> GSHLEPTQLGGLVTDQLARLCDVARLDRTDTETYVQTLATSLGTAAERSLALPPTTATLLSDDHTPVEYSLAFLPGATPALRVLVEPGWDSGDLAENGRAGLRAIRAMADRWNFSTDQLDLLEDLFFPVAPAGPFALWCALELRPGGVPGVKVYLNPAARGRDRRAETLREALDRLGHRQAFAALPPADDYPFLALDLGEWAAPRVKVYCTHESLSAQEAGEYSRLAAADGRDQTTDFFHAVAGTDAGGTGQPSTRRALTCHSFTDTVTGRPSGFTLHMPVRSYVEHDGRARDRAADVLRRYGMDNDALDRALAAVTPRPLDDGVGLVAYVALVHQLGRDPRVTVYVSSEAYAVQPPRTALA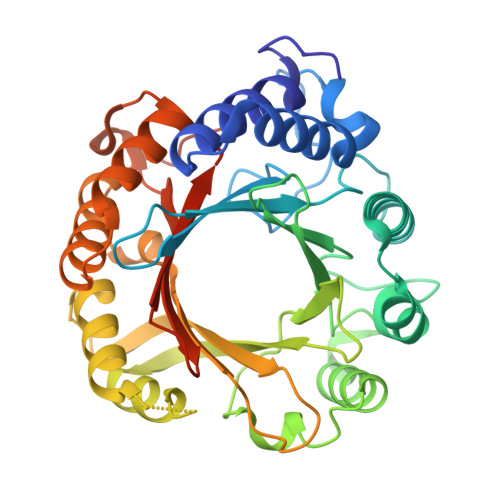TGPGIGR>[4x]MAEEKELVLLDFWVSPFGQRCRIA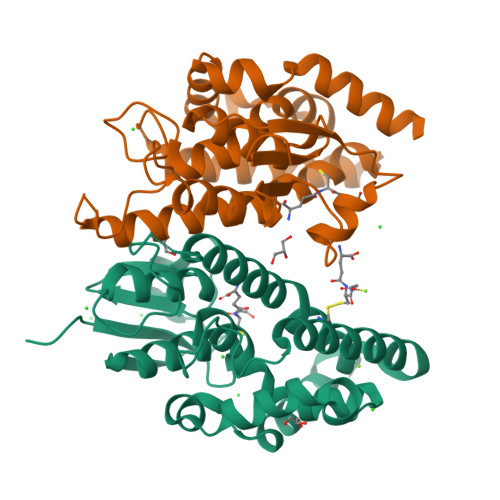MAEKGLEFEYREEDLGNKSDLLLRSNPVHRKIPVLLHAGRPVSESLVILQYLDDAFPGTPHLLPPANSGDADAAYARATARFWADYVDRKLYDCGSRLWRLKGEPQAAAGREMAEILRTLEAELGDREFFGGGGGGRLGFVDVALVPFTAWFYSYERCGGFSVEEVAPRLAAWARRCGRIDSVVKHLPSPEKVYDFVGVLKKKYGVE~{N}-[[1-[2-(~{tert}-butylamino)-2-oxidanylidene-ethyl]piperidin-4-yl]methyl]-3-chloranyl-5-fluoranyl-benzamide 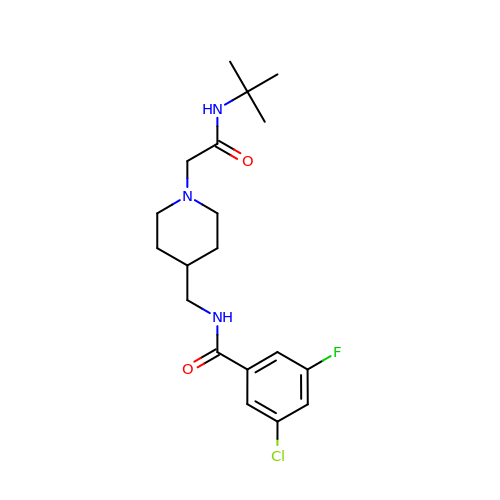| C19 H27 Cl F N3 O2 | JOCLITFYIMJMNK-UHFFFAOYSA-N> HHHHHHRAPPDKIAVIGAGIGGTSAAYYLRQKFGKDVQIDVFERGEVGGRLATLNVEGQEYEAGGSVIHPLNLHMKRFVKELGLSVSQGAGGLMGIYNGETFVFEESSWFIINVIKLLWHYGFQFLRMHMWVEDILDKFMRIYRYQSHDYAFSSVEGLLHALGGDEFTRMLNRTILEALQKAGFSQKFLNEIVTPAMRVNYGQSTNINGFVGAVSLAGADSGLWSVEGGNKLVCSGLLQASKARLISGSVTSIEEKTRTKQTGGTVKLYEVTYQTDSGTASDLYDIVVVATPLNRKMSNITFLNFNPPIPEFHKYYHQTVTTFVHGRLNASFFGYKAPDSFHLTDILTTDNPDLFINSIGVVSPVKEKADAASPPATGSAVWKVFSQEPLTKEQLNLLFASYDSVKEKKWLAYPHYKPPEKCPPIILHDRMYYLNGIEWAASAMEMSAIAAHNAALLAYHRWYGNTEMIDQEGLYEKLKTEL

Prenylcysteine oxidases (PCYOXs) metabolize prenylated cysteines produced by protein degradation. They utilize oxygen as a co-substrate to produce free cysteine, an aldehyde, and hydrogen peroxide through the unusual oxidation of a thioether bond. PCYOX1 contains a non-covalently bound flavin and metabolizes free prenylcysteine into cysteine, an isoprenoid aldehyde, and a stoichiometric amount of hydrogen peroxide. The resulting phylogeny clearly indicates that PCYOX1 and PCYOX1-like clades arose from a gene duplication event from a common ancestor at the emergence of Gnatosthomata about 460 million years ago.

As they show high sequence identities with their human counterparts (78% and 88%, respectively) they were selected for experimental characterization as models to understand the human proteins. Reflecting its high stability and operability, PCYOX1 could be crystallized, and its structure was solved at 3.1 Å resolution using AlphaFold2-predicted coordinates as a search model. PCYOX1, a monomeric protein, is composed of two domains: the classical dinucleotide-binding domain with the Rossmann motif and a specific prenylcysteine-oxidase domain. The FAD prosthetic group is bound to the Rossmann fold in an extended conformation. Beside this overall similarity, PCYOX1 is distinguished by the presence of a wide and elongated tunnel-shaped cavity extending orthogonally from the flavin ring to the protein surface. Computational docking predicts that the substrate binds with the isoprenoid tail extended along the cavity towards its entrance. However, a large hydrophobic patch is located on the underside of the enzyme. An electron density peak on this surface region convincingly matches the shape of the sterolic head of CHAPS, the detergent used for crystallization. This region likely represents the site of association of PCYOX1 to the membrane and may act synergistically with the KTEL C-terminal sequence to retain the protein in the endoplasmic reticulum. Notably, the entrance to the substrate binding cavity is adjacent to this hydrophobic patch.>ASQEISKSIYTCNDNQVMEVIYVNTEAGNAYAIISQVNEMIPMRLMKMASGANYEAID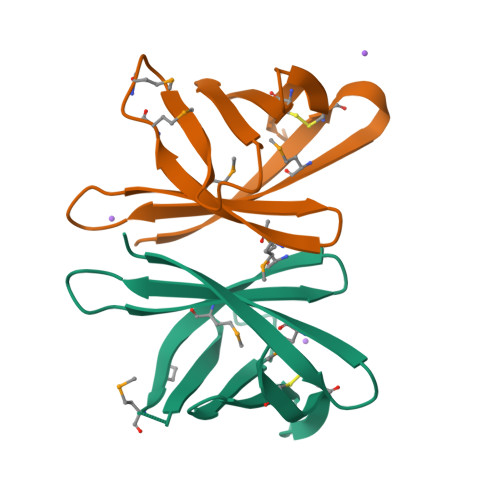KNYTYKLYTKGKTAELVEGDDKPVLSNCSLANLEHHHHHH[6x]>[2x]MASMTGGQQMGAPITAYAQQTRGLLGCIITSLTGRDKNQVEGEVQIVSTATQTFLATC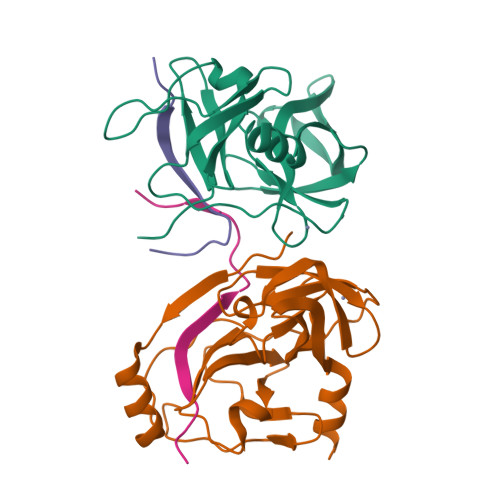INGVCWTVYHGAGTRTIASPKGPVIQMYTNVDQDLVGWPAPQGSRSLTPCTCGSSDLYLVTRHADVIPVRRRGDSRGSLLSPRPISYLKGSSGGPLLCPAGHAVGLFRAAVCTRGVAKAVDFIPVENLETTMRSGSHHHHHH;>[2x]KKGSVVIVGRIVLSGKPAIIPKK> MAYAQWVIIIIHNVGSQDVKIKNLKASWGKLHADGDKDAEVSASNYEGKIVKPDEKLQINASGRS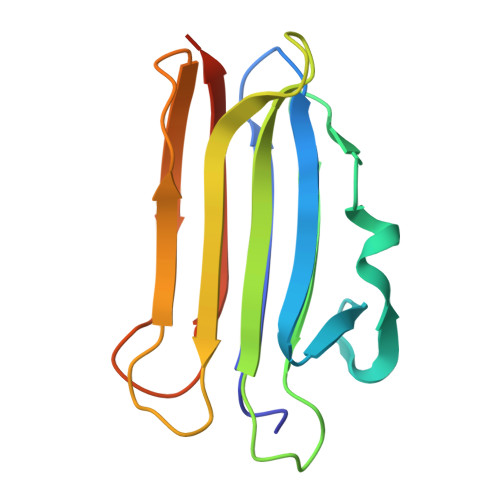DAAAGTTGTFDLVDPADGDKQVRHFYWDSPWGSKTNTWTVSGSNTKWMIEYSGQNLDSGALGTITVDTLKKGENLYFQ> ATETSFIIDAFNKTNLILQGDATVSSNGNLQLSYNSYDSMSRAFYSAPIQIRDSTTGNVASFDTNFTMNIRTHRQANSAVGLDFVLVPVQPESKGDTVTV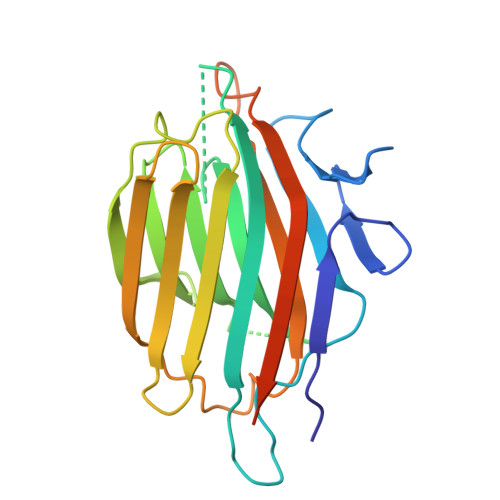EFDTFLSRISIDVNNNDIKSVPWDVHDYDGQNAEVRITYNSSTKVFSVSLSNPSTGKSNNVSTTVELEKEVYDWVSVGFSATSGAYQWSYETHDVLSWSFSSKFINLKDQKSERSNIVLNKIL> GQDEERDVGDDPFVRRAGAFLGIEAGTITIELSNLIDFYIRNGILEMENEQAVYPVNLRGVFDLNILQEMYRQYLIQSFAAKSRTEKERLFNNLAHLGNILGLTSAEVNAIHSNIGSVIYKTYASQALTNNRLEEKDIEFLRNIQNMLSMDEATCRTLLQETKEARAGFLFDKIFSRTFGMAEAVAEFRRVCRELDVDPVRDLKLTEDRRVRAFRAEIEHAIENGLITPENQSLLKESQEELGISAEKARQVLLDCIQDRCEALIVQAAASLRQRRQEGAARDLSRALRFGKLLPFQVQTPTVTGAERQELYLVYQAYALGTARSNAENDQVKEDLALLREMLGIQAA

Tic110 is an essential translocon component. Tic110 is therefore proposed to be the major channel for translocation of protein across the inner membrane. The second model also shows Tic110 with a membrane anchor composed of TM1 and TM2, but the rest of the protein is entirely soluble and localized in the stroma (Figure 1a, model 2; Inaba et al., 2005, 2003; Jackson et al., 1998). Tic110 is thus proposed to function as a scaffold in the stroma for binding transit peptides emerging from the inner-membrane channel, and for recruiting/tethering other translocon components located in the stroma. To investigate the structure of Tic110, we cloned and expressed the Tic110 homologue from Cyanidioschyzon merolae 10D, herein named CmTic110, for structural studies.

CmTic110C, composed of residues 871–1218, contains the corresponding region from the middle of TM5 to the C terminus. The crystal structure of CmTic110C was determined by selenium single-wavelength anomalous dispersion (Se-SAD) at a resolution of 4.2 Å. Our structure covers residues 903–1213, missing the first 32 and the last five residues of the CmTic110C construct. The structure comprises 14 α-helices of seven continuous anti-parallel helix-loop-helix pairs, forming an elongated shape of about 96 × 28 × 15 Å. Due to the low resolution, CmTic110C is assigned as a poly-Ala structure, except for the six Met residues. The region corresponding to TM6 consists of helix 3 and part of the loop connecting helix 4 in our structure (colored in yellow). This region is 28.2 Å high, much smaller than the 60–80 Å thickness observed for the chloroplast inner envelope membrane. Therefore, this helix is unlikely to cross the inner membrane. In the crystal packing, CmTic110C formed an extended superstructure with tail-to-tail and head-to-head packing. Therefore, the shape and structure of the Tic110 C-terminal region most likely also enable Tic110 to function as a scaffold for interacting with other proteins in the chloroplast translocon complex.> MRRRVVLCCQDVGSLLSSKHSVHSGIGYHERVFSRNLLYRRYPVVTVLPKAGFTVLDTKRWIASSGPPVTGSPLSPVTNPSLNVGTGGGEAVAMEGPLPVSYSPGSGVNGSLPVTSTAITAHCDVLSECVAKADELAVQLKAQNALSASAEILTQEGMEEFVEELKTSATNEMTALVKQMQTTPLLQRAGMHELRRTLYYTTSLKERDWLEEKQYTAAMRMLTVEVLRRDGDGVLSADDVLYVTTHVVTANFYNRHLWNRMEKSLLKFSNYENIDMSSVKAFSTRLFKTRRGCAKETLDIRRKVLLAMSRRVGVLANDFDLPSLLGVLQCYTVHDLTPFHLEPLAIRATNHVGDFTPHECATLAHVLRKWRTMRLEVCERLVERICTSDQLTHHMANAAMIAIRTCFNQVSDGGRNAMNAEPTRQKLRAMGEQIGCRLDEVEYPALPVILSILDVVVTLKIYVPKKCLQVIFSQANDMVAIVMEQKDDLVDPKTGKRVRPITAEEGRQLQALLS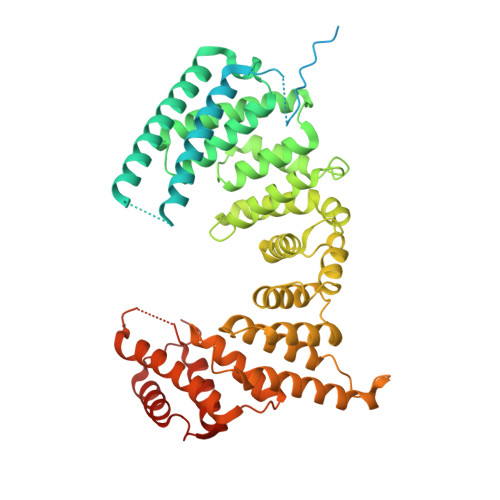HYGNDLAPELSQRMKEAFREGVLPDEASL>MAEAGITGTWYNQLGSTFIVTAGADGALTGTYESAVGNAESRYVLTGRYDSAPATDGSGTALGWTVAWKNNYRNAHSATTWSGQYVGGAEARINTQWLLTSGTTEANAXKSTLVGH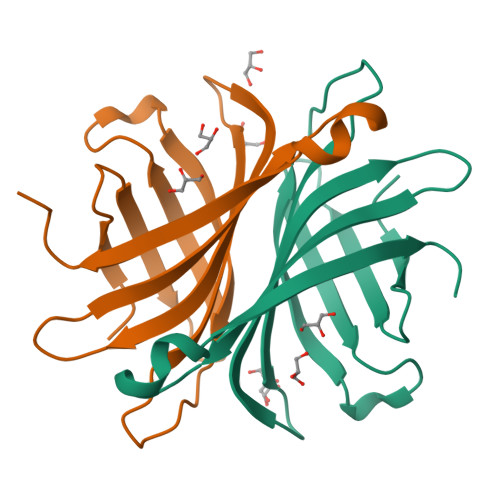DTFTKVKPSAASLEHHHHHH[2x]> QTAVTGGGASLPADLYKGSADSILPANFSYAVTGSGTGKKAFLENNSALFSTTGTVHFAGSDSVLSSTELNTYNSTYNVSGDANRYGALVQIPSVATSVTIPFNKAGSAVDLSVTQICGIFSGKINNWSQLAGLGR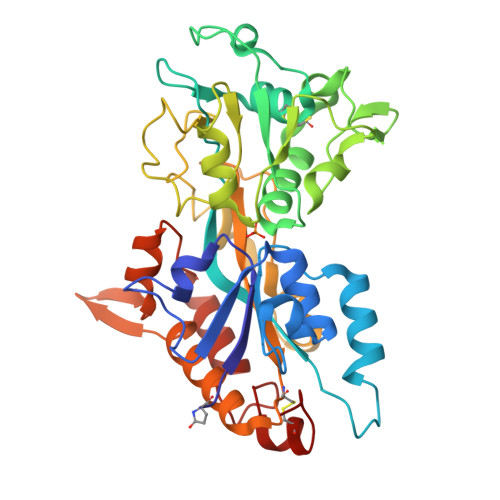TGAIQVVYRGESSGTSELLTRFLTSACQPADVSGTNLKLANGVPAFSVQSTFANLFTTVPSNFVAAPATGGSALYNAVYAVDGRVGYVGPDVIPSLTDATKVAKVKSFSPDEVSVQATLETAAPPTGAAAENPANWVPVFGNPSAGYPIAGYTNFVFGQCYKNATVGANVRGFLTRHYGSTVVNGVEQGPNDDAIRAHKFIPLTKAWRDAVRARFATATNAGAVNNPSTCSGIGRPL5-OXOHEXANOIC ACID | C6 H10 O3 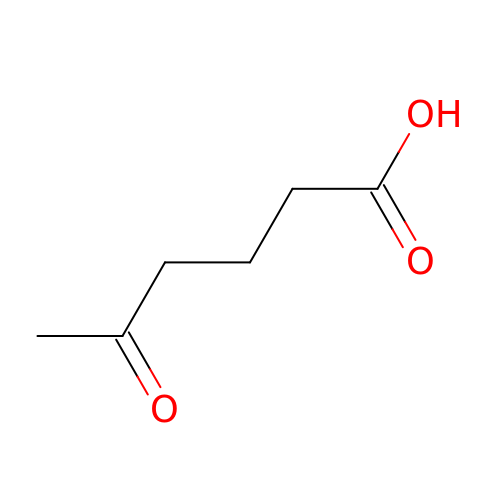| MGTZCLMLSSAXLD-UHFFFAOYSA-N>MAHTAAERPPEETLSLWKGEQARLKARVVDRDTEAWQRDPSFSGLQKVGGVDVSFVKGDSVRACASLVVLSYPELKVVYEDSRMVGLKAPYVSGFLAFREVPFLVELVQRLQEKEPDLMPQVVLVDGNGVLHQRGFGVACHLGVL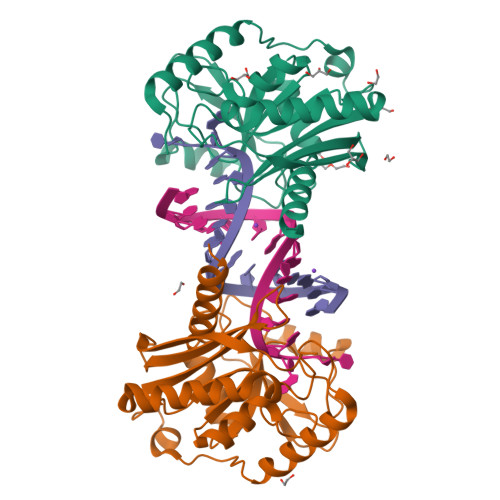TELPCIGVAKKLLQVDGLENNALHKEKIVLLQAGGDTFPLIGSSGTVLGMALRSHDHSTKPLYVSVGHRISLEVAVRLTHHCCRFRIPEPIRQADIRSREYIRRTLGQ[2x]> SNAMSEHKILARVPISVRWRDMDSMGHVNNAKYISYLEEARVRWMLGVEGVAMTDRIA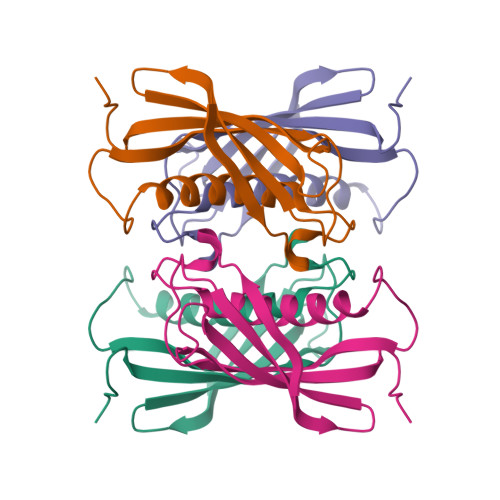PVVAATNVNYKRPLVWPNDILVELFVERLGSSSVTIGHRILDQKDEGVLYSDGNVVVVWIDTQTGKSASLPDAVRAASS Triosephosphate isomerase (TPI) interconverts glyceraldehyde 3-phosphate (G3P) and dihydroxyacetone phosphate (DHAP). One or various cytoplasmic and chloroplast TPIs (cTPI and pdTPI), are present in plant genomes. cTPIs are involved in glycolysis, whereas chloroplast enzymes participate in the Calvin-Benson cycle. The three-dimensional structures of AtTPIs confirm that both enzymes assembled as dimers with asymmetric units containing two monomers that fold into a canonical (β-α)8 or TIM-barrel. In conclusion, our data indicate that the duplicated TPI gene from A. thaliana has suffered two evolutionary fates: the cTPI isoform is susceptible to redox agents, whereas the pdTPI isoform is resistant.

Crystal structures of cTPI and pdTPI were solved at 1.7 and 2.15 Å respectively. Residue cTPI-C13 presents an ASA of 2.6 and 2.8 Å2 for monomers A and B respectively, whereas residue C218 presents an ASA of 6.7 and 2.6 Å2 for monomers A and B respectively. DTNB conjugation indicates that cTPI presents 2 accessible cysteines suggesting that both cTPI-C218 and cTPI-C13 are possible targets of redox agents. We found that the addition of 1 mM of DA inhibited cTPI activity to less than 5% of the untreated level, a response also observed in yeast TPI. At a GSSG concentration of 0.87 mM, using cTPI at 0.184 μM (10 μg/ml), enzymatic activity decreased to ~70% with respect to the activity of the untreated cTPI and was completely inhibited at concentrations above 6.5 mM. As expected, the glutathionylation signal was absent on the cTPI-C13S/C218S double mutant, indicating that in cTPI only residues C13 and C218 are glutathionylated and are potential targets of glutathionylation in vivo. Residue cTPI-C218 is located on α-helix 7, distant from the active site and the dimer interface. cTPI-C218S mutant exhibits a decrease in activity by more than 140-fold in comparison to wild-type cTPI activity. From these loop 3 residues, the only interaction that is different between AtTPIs, is that in cTPI residue M83 makes a hydrophobic interaction with cTPI-C13, whereas in pdTPI residue Q83 makes a H-bond with pdTPI-C15. Residue cTPI-C218 is the most exposed cysteine in cTPI, in contrast pdTPI presents a serine at this position (pdTPI-S218). cTPI-C218 and pdTPI-S218 are surrounded by charged amino acids. However, cTPI-C218 is located before a lysine, whereas pdTPI-S218 is positioned before an alanine indicating that the epsilon amino group of cTPI-K219 may contribute to the reactivity of cTPI-C218.

>[2x]GPHMARKFFVGGNWKCNGTAEEVKKIVNTLNEAQVPSQDVVEVVVSPPYVFLPLVKSTLRSDFFVAAQNCWVKKGGAFTGEVSAEMLVNLDIPWVILGHSERRAILNESSEFVGDKVAYALAQGLKVIACVGETLEEREAGSTMDVVAAQTKAIADRVTNWSNVVIAYEPVWAIGTGKVASPAQAQEVHDELRKWLAKNVSADVAATTRIIYGGSVNGGNCKELGGQADVDGFLVGGASLKPEFIDIIKAAEVKKSA ACRYLIC ACID | C3 H4 O2 | 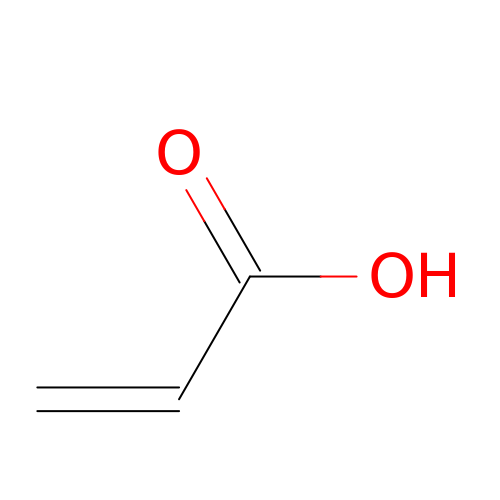NIXOWILDQLNWCW-UHFFFAOYSA-N Diagnostic testing and symptomatic treatment of myasthenia gravis are based on restoration of cholinergic transmission at the neuromuscular junction by means of peripherally-acting inhibitors of acetylcholinesterase (AChE), the enzyme responsible for the hydrolysis of the neurotransmitter acetylcholine at the synapse. Inhibition of acetylcholine breakdown renders the neurotransmitter more available for nicotinic AChR stimulation, which alleviates muscle weakness by improving neuromuscular transmission. In this study, we explored two different approaches to accessing more polar derivatives of tacrine, 6-chlorotacrine, and huprine Y, which may serve as new peripherally-acting AChEIs of potential value for treatment of myasthenia gravis. Furthermore, the three-dimensional structures of complexes of several of these compounds with Torpedo californica AChE (TcAChE) were also solved, in order to shed light on their mechanism of action.

In the crystal structure of TcAChE complexed with the 6-chlorotacrine-based triazole derivative 16, the 6-chlorotacrine moiety binds as previously observed, with the conjugated system π-stacked to Trp84, and the Cl atom fitting into the hydrophobic groove comprising Phe330, Tyr334, Trp432, Met437, and Ile439. Along the linker, the triazole ring is engaged in two perpendicular π-stacking interactions with Tyr334 and Phe300, and in H-bonds with Tyr121 and Asp72. From this point onwards, the observed conformations of the phenolic moiety of 16 differ in the two TcAChE monomers of the asymmetric unit. In monomer A, the phenolic moiety makes a π-stacking interaction with Trp279 in the PAS. In monomer B, the ether oxygen of the phenolic moiety H-bonds to the main carbonyl of Arg289. In general, these structural changes lead to decreased AChE and BChE inhibitory activities relative to the parent compounds, with the exception of the triazole-containing compound 16, which is a more potent AChE and BChE inhibitor than the parent 6-chlorotacrine, likely as a result of multi-site binding within the active-site gorge of the enzyme, as confirmed by the crystal structure of its complex with TcAChE. In this context, the huprine and triazole derivatives 6, 10 and 16 are those with the most potent and selective hAChE inhibitory activity, with IC50 values of 59.2 nM, 200 nM and 7.18 nM, respectively, and selectivities for hAChE over hBChE inhibition of 55, 16, and 40, respectively. Most important, these compounds are 23-, 7- and 192-fold more potent and 37-, 11- and 27-fold more selective hAChE inhibitors than pyridostigmine, the most widely used drug for treatment of myasthenia gravis and other myasthenic syndromes.

>[2x]DDHSELLVNTKSGKVMGTRVPVLSSHISAFLGIPFAEPPVGNMRFRRPEPKKPWSGVWNASTYPNNCQQYVDEQFPGFSGSEMWNPNREMSEDCLYLNIWVPSPRPKSTTVMVWIYGGGFYSGSSTLDVYNGKYLAYTEEVVLVSLSYRVGAFGFLALHGSQEAPGNVGLLDQRMALQWVHDNIQFFGGDPKTVTIFGESAGGASVGMHILSPGSRDLFRRAILQSGSPNCPWASVSVAEGRRRAVELGRNLNCNLNSDEELIHCLREKKPQELIDVEWNVLPFDSIFRFSFVPVIDGEFFPTSLESMLNSGNFKKTQILLGVNKDEGSFFLLYGAPGFSKDSESKISREDFMSGVKLSVPHANDLGLDAVTLQYTDWMDDNNGIKNRDGLDDIVGDHNVICPLMHFVNKYTKFGNGTYLYFFNHRASNLVWPEWMGVIHGYEIEFVFGLPLVKELNYTAEEEALSRRIMHYWATFAKTGNPNEPHSQESKWPLFTTKEQKFIDLNTEPMKVHQRLRVQMCVFWNQFLPKLLNATACDGELSSSGTSSSKGIIFYVLFSILYLIF>[6x]MAVEPFPRRPITRPHASIEVDTSGIGGSAGSSEKVFCLIGQAEGGEPNTVYELRNYSQAKRLFRSGELLDAIELAWGSNPNYTAGRILAMRIEDAKPASAEIGGLKITSKIYGNVANNIQVGLEKNTLSDSLRLRVIFQDDRFNEVYDNIGNIFTIKYKGEEANATFSVEHDEETQKASRLVLKVGDQEVKSYDLTGGAYDYTNAIITDINQLPDFEAKLSPFGDKNLESSKLDKIENANIKDKAVYVKAVFGDLEKQTAYNGIVSFEQLNAEGEVPSNVEVEAGEESATVTATSPIKTIEPFELTKLKGGTN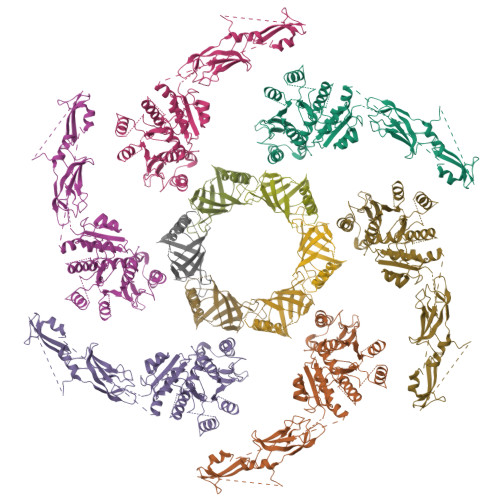GEPPATWADKLDKFAHEGGYYIVPLSSKQSVHAEVASFVKERSDAGEPMRAIVGGGFNESKEQLFGRQASLSNPRVSLVANSGTFVMDDGRKNHVPAYMVAVALGGLASGLEIGESITFKPLRVSSLDQIYESIDLDELNENGIISIEFVRNRTNTFFRIVDDVTTFNDKSDPVKAEMAVGEANDFLVSELKVQLEDQFIGTRTINTSASIIKDFIQSYLGRKKRDNEIQDFPAEDVQVIVEGNEARISMTVYPIRSFKKISVSLVYKQQTLQA;>[6x]MALKAQNTISGKEGRLFLDGEEMAHIKTFEANVEKNKSEVNIMGRRMTGHKTTGANGTGTATFYKVTSKFVLLMMDYVKKGSDPYFTLQAVLDDQSSGRGTERVTLYDVNFDSAKIASLDVDSEALEEEVPFTFEDFDVPEKLSDTFLEHHHHHH> MHHHHHHGSEFMASDQVTLLDFWPSPFGMRVRLALAEKGVKYEYSEEDLRNKSALLLQMNPVNKQIPVLVHNGKPVCESLIIVQYIDEVWKDSAPLLPSDPYQRAQSRFWADFVDKKIYDLGRKIWTKKGEEQEAAKKDFIDSLKLMEGELGDKPYFGGETIGYVDIALVPFYSWFYAYE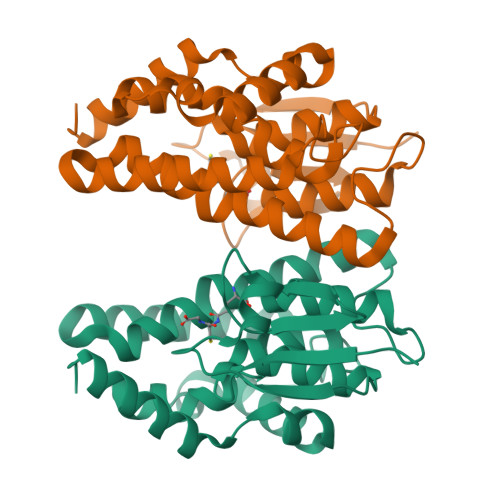TIGNFNIEAECPKMIAYCKRCLQKETVSKALEDPQKVYDFVLMLMKKFGIE>GHMTGIPSIVPYALPTSRDLPANLAQWHIDPERAVLLVHAMQRYFLRPLPDALRDQVVGNAARIRQWAADNGVPVAYTAQPGSMNEEQRGLLKDFWGPGMKASPTDREVVDALAPQPGDWLLTKWRYSAFFNSDLLQRLHASGRDQLILCGVYAHVGVLISSVDAYSNDIQPFLVADAIADFSKEHHWMAME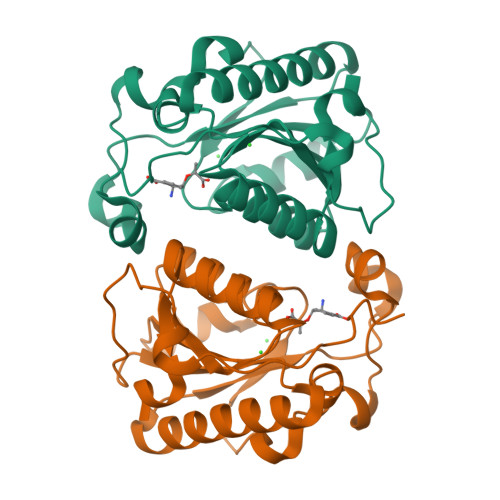YAASRCAMVITTDEVVL[2x]>ATMQPFHSPEESVNSQFYLPPPPGNDDPAFRYDKEAYFKGYAIKGSPRWKQAAEDADISVENIARIFSPVVGAKISPKDTPETWNMLQNLLKVGGYYATASAKKYYMRTRPFVLFNHSTCRPEDENTLRKDGSYPSGHTAYSTL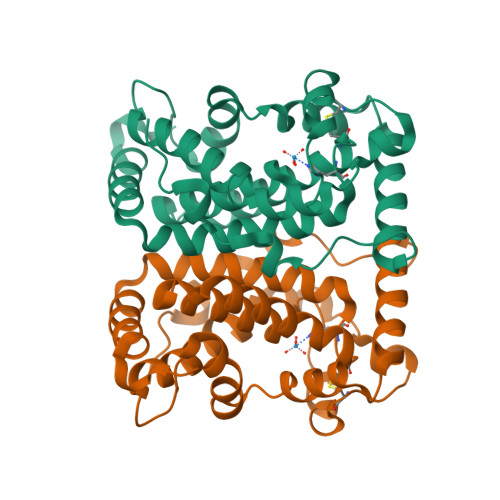LALVLSQARPERAQELARRGWEFGQSRVICGAHWQSDVDAGRYVGAVEFARLQTIPAFQKSLAKVREELNDKNNLLSKEERPELNY[4x]>MQPINTSNPDNTASYVKDEVEITSSTIALSEIVSVVNTSDGRLEVFGVGTDKAVWHNRQMAPHTGSPWSGWSSLKGQVTSKPVVYINTDGRLEVFARGTDNALWHIWQTATNAGWSNWQSLGGVITSNPAIYANTDGRLEVFARGADNALWHISQTTAHSGPWSSWASLNGVITSNPTVHINSDGRLEVFARGTDNALWHIWQTAPDSNLWSSWESLNGIITSDPVVIDTADGRLEVFARGADNALWHIWQTISHSGPWSGWQSLNGVITSAPAVAKNCDNRLEAFARGTDNALWHTWQTVSHSGPWSSWQSLNGVITSAPTAVRDADGRLEVFARGTDNALWLTWQTASSWSPWISLGGVLIDASAIK[2x]

As a part of our ongoing programme focused on host-pathogen interactions at the molecular level, we identified a lectin in the P. asymbiotica genome designated PHL, which we prepared in a fully functional recombinant form. The lectin PHL interacts selectively, mainly with l-fucose and oligosaccharides containing terminal l-fucose residue, and prefers an α-glycosidic bond over a β-linkage. The PHL lectin forms a seven-bladed β-propeller assembling into a homo-dimer. Both units contain two types of binding sites situated between the blades and have different amino acid compositions and binding preferences.

As mixing PHL with the branched compounds leads to protein precipitation and thus prevents co-crystallization, the direct study of complexes was not possible. Therefore, we soaked the PHL crystals with monomeric fucoside 2, 3 and 4, respectively. Crystal structures confirmed that all the studied fucosides were able to bind the lectin PHL. In each complex, the electron density was clear enough to determine the position of the fucosyl part of the compounds in 6 out of 7 fucose-binding sites of at least one PHL monomer unit – A or B, while site 2 is occupied by Met60 of the neighbouring monomer, as was observed previously. The second saccharide unit was clearly assigned for all three fucosides 2–4 in sites 1 and 3. For fucoside 3 and 4, the second saccharide was also distinguishable in sites 4-7 of at least one protein monomer. Considering fucosides 2–4, the position of the bridging methylene group is close to the α-Me-Fuc O1 atom, which is not directly coordinated by the protein in the complex. The O4 of the d-arabino-hexopyranosyl unit in fucoside 2 and 4 is coordinated by a glycine backbone nitrogen in sites 1, 3, 5, and 6, while the O6 atom of fucoside 3 is linked to a tryptophan backbone oxygen in sites 4 and 6. When comparing the overall orientation of the second hexopyranosyl unit of fucosides 2–4, it is similar to the galactose unit of blood group H trisaccharide, with minor distortions in individual binding sites influenced e.g. by crystal packing. The second saccharide unit of studied fucosides was only marginally coordinated by PHL binding sites what, together with affinity comparable to monosaccharides, suggests a low importance of this type of compounds for inhibitor design.>GSGPPGPPGPPGPPGARGEPGNIGFPGPPGPPGPPGRAPTDQHIKQVCMRVIQEHFAEMAASLKRPDSGAT[2x];>[2x]GSGPPGPPGPPGPPGARGQAGVMGFPGPPGPPGPPGRDATDQHIVDVALKMLQEQLAEVAVSAKREALGAV;>GSGPPGPPGPPGPPGARGQAGVMGFPGPPGPPGPPGKEASEQRIRELCGGMISEQIAQLAAH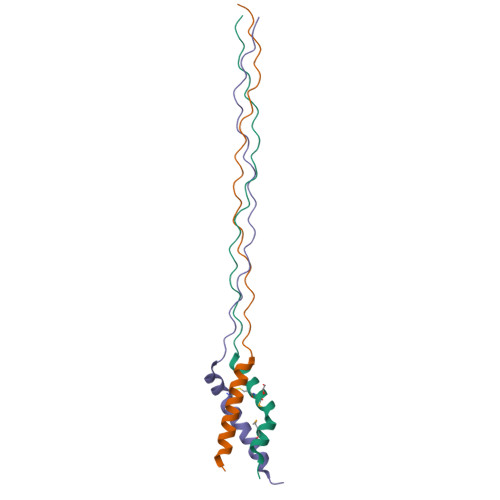LRKPLAPGSI[2x]HETEROARYLALANINE 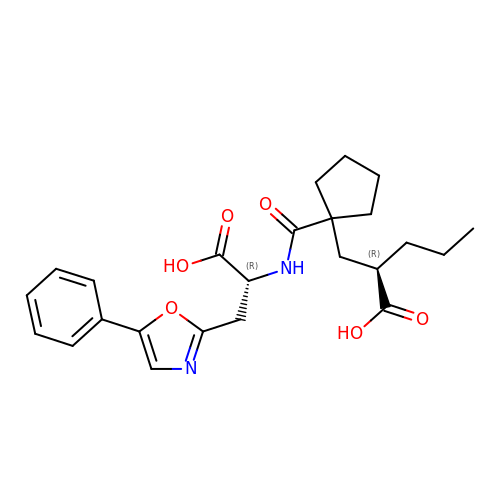5-PHENYL OXAZOLE | C24 H30 N2 O6 | SFZJKCPBOHKUKC-QZTJIDSGSA-N>[3x]MAQVVRQKFKDVTTE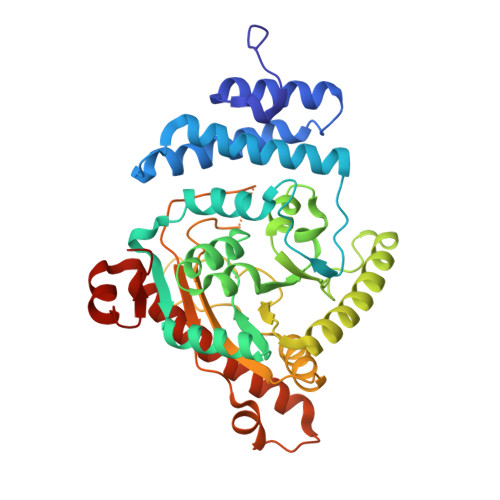QEFFAVLQDEIAQGHVPKLLMPAFQDFYNNYKTAVLGSGVPGADEALVAKIMSAIADRSVHEFVEPYTFPSFHHRILEPYNYYQFGQNYVRTLLDFSKSVVGHLARFDEIEQQIAAGENVVLLANHQTEADPGVFALLLEHTHPRLATDVIYVAGDRVVTDPLCKPFSMGRNLFCVHSKKRLDDIPELKASKVATNRRTLSAMTKALNEGGRLLWIAPSGGRDRPQADTGAWHPDKFDPTAVELMRQLLSRSAPKGHLYPFAMYSWELMPPPKGVEKGLGERRLTHFAGTGISVCKELDVDSIVSSAAVEDKATRQQLLATAAWQAVSDEYAILEEVIGSEDARRQRSDVYQQPWAQ>MPLCTLRQMLGEARKHKYGVGAFNVNNMEQIQGIMKAVVQLKSPVILQCSRGALKYSDMIYLKKLCEAALEKHPDIPICIHLDHGDTLESVKMAIDLGFSSVMIDASHHPFDENVRITKEVVAYAHARSVSVEAELGT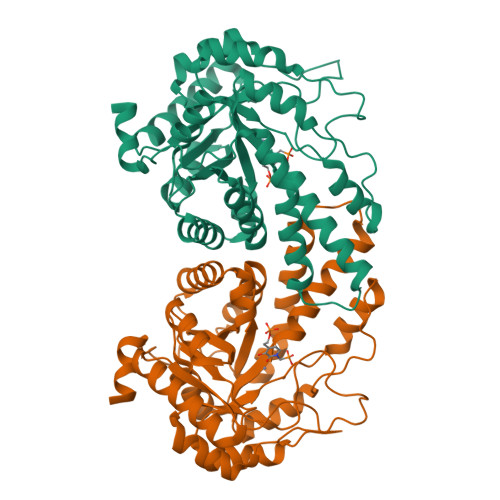LGGIEEDVQNTVQLTEPQDAKKFVELTGVDALAVAIGTSHGAYKFKSESDIRLAIDRVKTISDLTGIPLVMHGSSSVPKDVKDMINKYGGKMPDAVGVPIESIVHAIGEGVCKINVDSDSRMAMTGAIRKVFVEHPEKFDPRDYLGPGRDAITEMLIPKIKAFGSAGHAGDYKVVSLEEAKAWYK[2x]> MGHHHHHHHHAIAENLYFQSAAGLHISDGRLVEGNGNDFVMRGINHAHTWYPGETQSLADIKATGANTVRVVLSDGYRWSE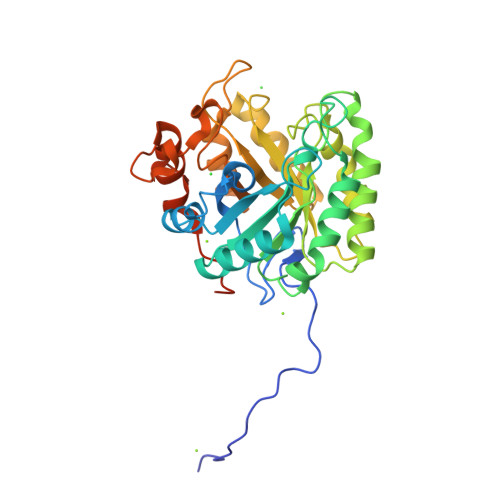NSPEDVASIIARCKAERLICVLEVHDTTGYGEDAAAGTLDHAADYWIGLKDVLDGEEDYVVINIGNEPWGNADPAGWTAPTTAAIQKLRAAGFAHTIMVDAPNWGQDWEGVMRADARSVYDADPTGNLIFSIHMYSVYDTAAKVTDYLNAFVDAGLPLLIGEFGGPADQYGDPDEDTMMATAEELGLGYLAWSWSGNTDPVLDLVLDFDPTRLSSWGERVLHGPDGITETSREATVFGGGQGGGDTEAPTAPGTPT>[2x]SDVFHLGLTKND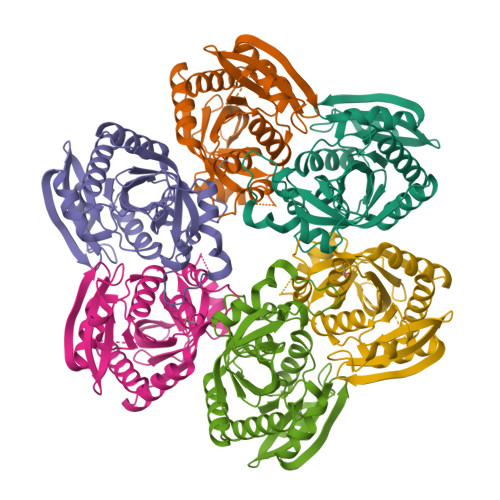LQGAQLAIVPGDPERVEKIAALMDKPVKLASHREFTSWRAELDGKAVIVCSTGIGGPSTSIAVEELAQLGIRTFLRIGTTGAIQPHINVGDVLVTTASVRLDGASLHFAPMEFPAVADFACTTALVEAAKSIGATTHVGVTASSDTFYPGQERYDTYSGRVVRRFKGSMEEWQAMGVMNYEMESATLLTMCASQGLRAGMVAGVIVNRTQQEIPNAETMKQTESHAVKIVVEAARRLL4-[4-({[3-tert-butyl-1-(quinolin-6-yl)-1H-pyrazol-5-yl]carbamoyl}amino)-3-fluorophenoxy]-N-methylpyridine-2-carboxamide 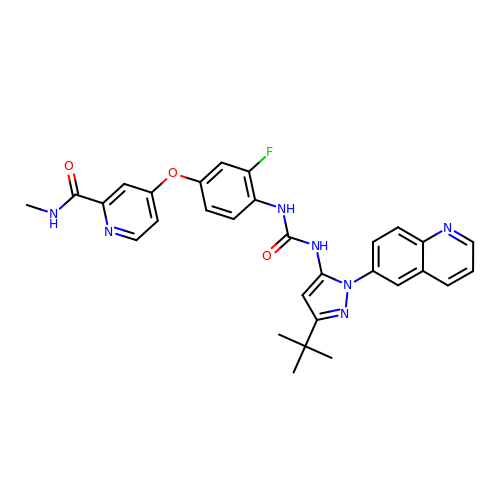| C30 H28 F N7 O3 | WVXNSAVVKYZVOE-UHFFFAOYSA-N> MASMTGGQQMGRDPNSMKNIESLFD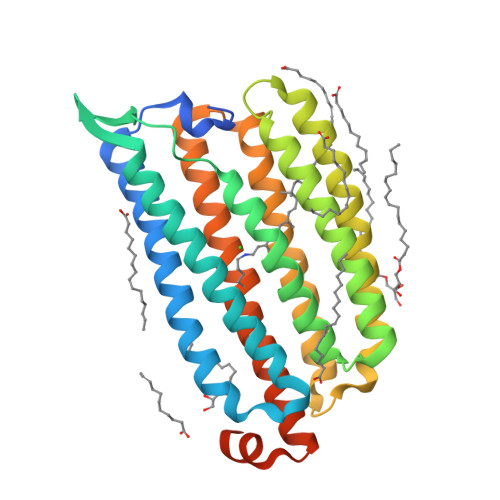YSAGQFEFIDHLLTMGVGVHFAALIFFLVVSQFVAPKYRIATALSCIVMVSAGLILNSQAVMWTDAYAYVDGSYQLQDLTFSNGYRYVNWMATIPCLLLQLLIVLNLKGKELFSTATWLILAAWGMIITGYVGQLYEVDDIAQLMIWGAVSTAFFVVMNWIVGTKIFKNRATMLGGTDSTITKVFWLMMFAWTLYPIAYLVPAFMNNADGVVLRQLLFTIADISSKVIYGLMITYIAIQQSAAAGYVPAQQALGRIGMDSKAALEHHHHHH A multiprotein complex in the outer membrane called β-Barrel Assembly Machine (BAM) then mediates OMP folding and insertion. In E. coli, the BAM complex is composed of BamA, a β-barrel OMP itself previously known as Omp85/YaeT, and the lipoproteins BamB, C, D and E (previously YfgL, NlpB, YfiO and SmpA respectively). BamB is a membrane-associated lipoprotein with lipids attached to the N-terminal cysteine in the mature protein predicted to anchor it to the membrane. Taken together, the structural analysis and mutagenic testing of BamB suggests that its main function is to bind and modulate BamA, rather than directly interact with nascent OMPs.

We report the crystal structure of Pseudomonas aeruginosa BamB refined to 1.85Å resolution. A lipid-free, soluble form of mature Pseudomonas aeruginosa BamB (paBamA, amino acids 19–380) was expressed in E. coli, purified to homogeneity and crystallized as described in Methods. The crystals belong to trigonal space group P3221 and contain a single paBamB molecule per asymmetric unit. The model was then refined against a native dataset to 1.85Å resolution. The final model contains amino acids 28 to 380 (plus two extra amino acids, PG, at the C-terminus resulting from the cloning procedure) with excellent refinement statistics as shown in Table 1. BamB adopts an eight-bladed β-propeller fold. Four antiparallel β-strands named A–D constitute each blade with the A strand being closest to the pseudo-symmetry axis (A1 thus refers to the A strand of Blade1). The eighth blade is formed by three strands from the C-terminus and the D-strand from the N-terminus (blue in Figure 1) mediating closure of the ring. Despite these irregularities in the inner strands, the propeller displays a central pore that is about 20Å wide at the “top” and narrows to about 8Å at the center. The structures of paBamB and ecBamB (E. coli BamB) superimpose with an RMS deviation of 1.8 Å for 286 matching Cα atoms highlighting a high degree of structural conservation despite a relatively modest 30% sequence identity.

> GAMASSNSKKELPPAELTDFKEEVVLSKQWSRSVGDGQGDLYNLLEPAVDGSTIYAASAEGRVMAIQRETGDVLWKKDLERPVSGGVGVGYGLVLVGTLRGDVIALDEATGKKKWTKRVNSEVLSAPATNGDVVVVQTQDDKLIGLDAASGDQRWIYESTVPVLTLRGTGAPLIAGNMALAGLASGKVVAVDVQRGLPIWEQRVAIPQGRSELDRVVDIDGGLLLSGDTLYVVSYQGRAAALDVNSGRLLWQREASSYVGVAEGFGNIYVSQASGSVEGLDSRGASSLWNNDALARRQLSAPAVFSSNVVVGDLEGYVHLLSQVDGRFVGRERVDSDGVRVRPLVVGSWMYVFGNGGKLVAYTIRPG>[2x]SNAMLKREMNIADYDAELWQAMEQEKVRQEEHIELIASENYTSPRVMQAQGSQLTNKYAEGYPGKRYYGGCEYVDVVEQLAIDRAKELFGADYANVQPHSGSQANFAVYTALLQPGD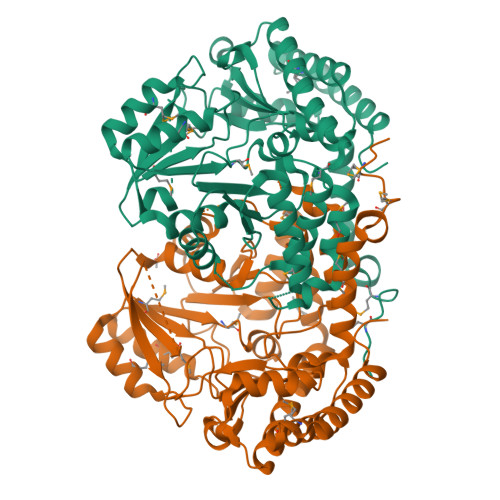TVLGMNLAQGGHLTHGSPVNFSGKLYNIVPYGIDESGKIDYDEMAKLAKEHKPKMIIGGFSAYSGVVDWAKMREIADSIGAYLFVDMAHVAGLIAAGVYPNPVPHAHVVTTTTHKTLAGPRGGLILAKGGDEELYKKLNSAVFPSAQGGPLMHVIAGKAVALKEAMEPEFKVYQQQVAKNAKAMVEVFLNRGYKVVSGGTENHLFLLDLVDKNLTGKEADAALGRANITVNKNSVPNDPKSPFVTSGIRIGSPAVTRRGFKEAEVKELAGWMCDVLDNINDEATIERVKAKVLDICARFPVYA Nucleoside diphosphate kinase A (NME1) is a multifunctional enzyme that was found to be pyrophosphorylated on Thr94 in human cells. A major role of NME1 is the synthesis of nucleoside triphosphates, other than ATP. NME1 catalyses this process by transferring the γ-phosphoryl group from ATP to a nucleoside diphosphate (NDP) via an active-site phosphohistidine intermediate. Oligophosphorylation was critically dependent on the catalytic histidine residue His118, and cryogenic electron microscopy analysis of the modified proteins suggests an intramolecular phosphoryl transfer mechanism.

Next, we investigated the structural aspects of NME1 in oligophosphorylated states and treated purified ppS94-NME1 with ATP to generate a heterogeneous mixture of oligophosphorylated NME1 for subsequent vitrification and cryo-EM data collection. The hexameric structure remained unaltered, even in these putatively oligophosphorylated states. Although heterogeneity posed a challenge in visualizing individual oligophosphorylation states, a larger density around ppS94 was identified. We were able to verify that this density corresponds to the pppS94 species localized at Ser94, with a likely further decrease in distance between His118 and the terminal phosphate. To visualize individual higher oligophosphorylation states in the heterogeneous dataset, symmetry expansion and focused three-dimensional (3D) classification of the phosphorylation site of one subunit were applied. This analysis revealed three subsets with different extents of cryo-EM density appearing around ppSer94, which is indicative of the presence of different chain-length oligophosphates. Class 1 contained 37% of sorted particles and exhibited only little additional density, which probably corresponds to pppSer94 in a different orientation, whereas class 2 (32% of particles) and class 3 (31% of particles) had larger densities, possibly indicative of higher phosphorylation states. Furthermore, class 3 showed a connection between the additional density found for the oligophosphate chain and the density for the loop consisting of residues Lys65–Phe61, which includes the positively charged Arg58 that could interact with the negatively charged oligophosphates. Oligophosphorylated NME1 displayed a notable amount of cryo-EM density at the surface of the NME1 hexamer, and it seems plausible that oligophosphorylation could act as a recruiting element to engage a different set of NME1 interaction partners. Next, the impact of oligophosphorylation on protein–protein interactions was explored using oligo-pS94-NME1, which was generated by treating ppS94-NME1 with ATP.

>MHHHHHHMANCERTFIAIKPDGVQRGLVGEIIKRFEQKGFRLVGLKFMQASEDLLKEHYVDLKDRPFFAGLVKYMHSGPVVAMVWEGLNVVKTGRVMLGESNPADSKPGTIRGDFCIQVGRNIIHGSDSVESAEKEIGLWFHPEELVDYT[6x]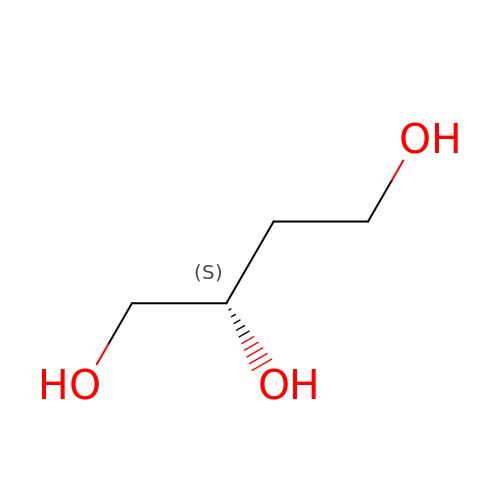(2~{S})-butane-1,2,4-triol | C4 H10 O3 | ARXKVVRQIIOZGF-BYPYZUCNSA-N>MVPISPIETVPVKLKPGMDGPKVKQWPLTEEKIKALVEICTEMEKEGKISKIGPENPYNTPVFAIKKKDSTKWRKLVDFRELNKRTQDFWEVQLGIPHPAGLKKKKSVTVLDVGDAYFSVPLDEDFRKYTAFTIPSINNETPGIRYQYNVLPQGWKGSPAIFQSSMTKILEPFKKQNPDIVIYQYMDDLYVGSDLEIGQHRTKIEELRQHLLRWGLTTPDKKHQKEPPFLWMGYELHPDKWTVQPIVLPEKDSWTVNDIQKLVGKLNWASQIYPGIKVRQLCKLLRGTKALTEVIPLTEEAELELAENREILKEPVHGVYYDPSKDLIAEIQKQGQGQWTYQIYQEPFKNLKTGKYARMRGAHTNDVKQLTEAVQKITTESIVIWGKTPKFKLPIQKETWETWWTEYWQATWIPEWEFVNTPPLVKLWYQLEKEPIVGAETFYVDGAANRETKLGKAGYVTNKGRQKVVPLTNTTNQKTELQAIYLALQDSGLEVNIVTDSQYALGIIQAQPDKSESELVNQIIEQLIKKEKVYLAWVPAHKGIGGNEQVDKLVS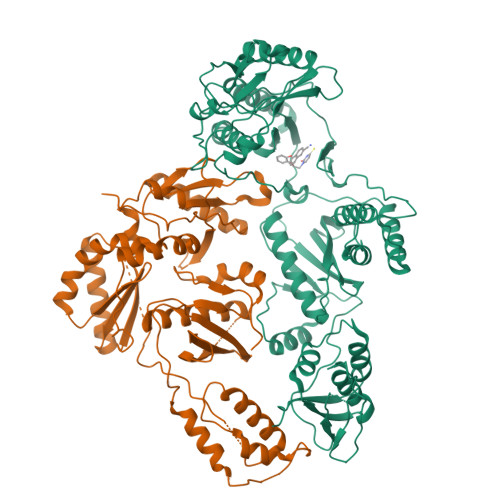AGENLYFQ[2x]4-OXO-NICOTINAMIDE-ADENINE 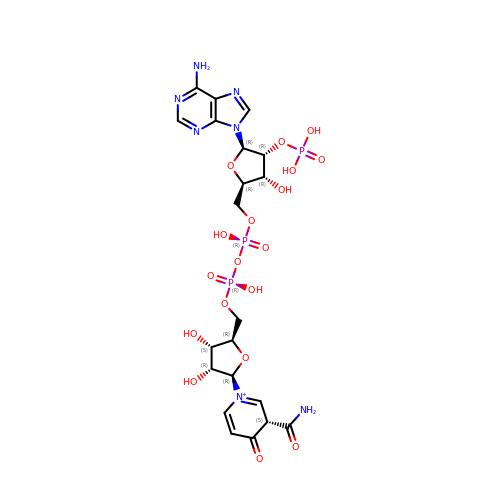DINUCLEOTIDE PHOSPHATE | C21 H29 N7 O18 P3 | PIXSDSMVQQICPA-BYJCYCELSA-O> MSAKPQPIAAANWKCNGTTASIEKLVQVFNEHTISHDVQCVVAPTFVHIPLVQAKLRNPKYVISAQNAIAKSGAFTGEVSMPILKDIGVHWVILGHSERRTYYGETDEIVAQKVSEACKQGFMVIACIGETLQQREANQTAKVVLSQTSAIAAKLTKDAWNQVVLAYEPVWAIGTGKVATPEQAQEVHLLLRKWVSENIGTDVAAKLRILYGGSVNAANAATLYAKPDINGFLVGGASLKPEFRDIIDATR

Triosephosphate isomerase (TIM) is a key enzyme in glycolysis that catalyses the interconversion of glyceraldehyde 3-phosphate and dihydroxy­acetone phosphate. The catalytic power of TIM is thought to stem from its ability to facilitate the deprotonation of a carbon next to a carbonyl group to generate an enediolate intermediate. Asn11 and Lys13 provide electrostatic stabilization, and together with His95 form an oxyanion-hole-like environment for the intermediates. Glu167 is thought to act as the catalytic base in the initial, rate-limiting proton-abstraction step to generate an enediolate intermediate, which is further stabilized by other residues in the active site.

Therefore, mechanism-based inhibitors that mimic the enediolate and enediol intermediates need to be used for structural studies. 2-Phosphoglycolate (PGA) has been considered to be a mimic of the enediolate intermediate and has a K i of 26 µM, having a much higher affinity than DHAP, which has a K m of 300 µM for LmTIM. Elegant studies by the John Richard group on the protonation state of the Glu167 side chain show that the pK changes from ∼4 to ∼10 when forming a complex with PGA, mimicking the protonation event of this glutamate upon substrate binding. The structures show that in the PGA complex the postulated general base Glu167 is protonated, while in the PGH complex it remains deprotonated. The differences between the room-temperature structure and the 1.19 Å resolution structure of the perdeuterated protein at 100 K are also small, with an all-atom r.m.s.d. of 0.12 Å. Moreover, none of the residues in the active site show any significant geometric changes between the room-temperature and 100 K structures. The atomic resolution structure of LmTIM with PGA shows a hydrogen bond of 2.61 Å between the carboxylate group of the inhibitor and Glu167.> MSAPGAGESRLGRPAPVMEREHDRPAALDHPRAPRKPRGIPYFEKYAWLFMRFSGIALVFLALGHLFIMLMWQDGVYRIDFNYVAERWASPFWQIWDMA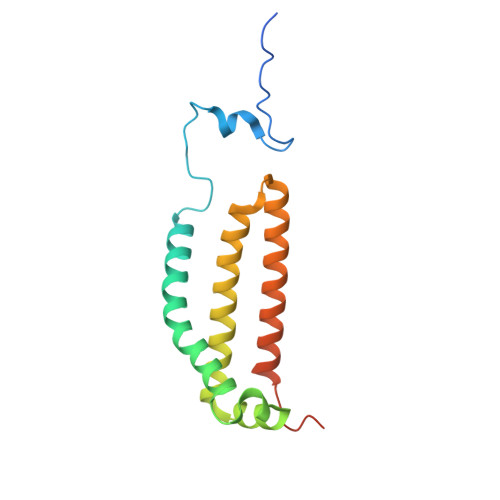LLWLAMIHGANGMRTIIGDYARKNVTKFWLNSLLLLATGFTLVLGSYVLVTFDANISHHHHHHHHHH>[4x]QNSHMVKDLNLYAKELVDVVNYLMKKNQLVFSRNNKFIYVNT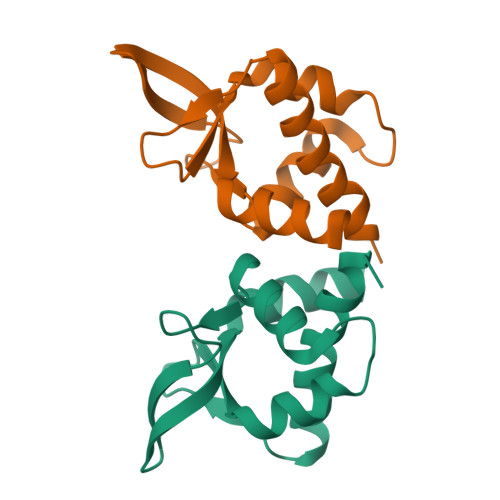ETIKSMLEKRNYDTVDGKLYLWRELEWIECAEDRFNKRIKIDGENMYAVVIKYSSYSILKRLYLE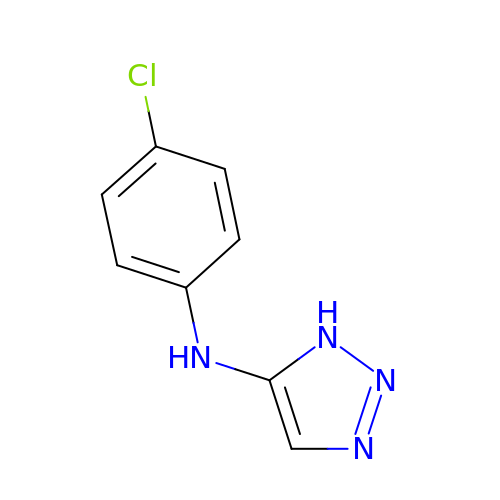~{N}-(4-chlorophenyl)-1~{H}-1,2,3-triazol-5-amine | C8 H7 Cl N4 | IUTZKZLVPUPHDA-UHFFFAOYSA-N> MSTLIPPPSKKQKKEAQLPREVAIIPKDLPNVSIKFQALDTGDNVGGALRVPGAISEKQLEELLNQLNGTSDDPVPYTFSCTIQGKKASDPVKTIDITDNLYSSLIKPGYNSTEDQITLLYTPRAVFKVKPVTRSSSAIAGHGSTILCSAFAPHTSSRMVTGAGDNTARIWDCDTQTPMHTLKGHYNWVLCVSWSPDGEVIATGSMDNTIRLWDPKSGQCLGDALRGHSKWITSLSWEPIHLVKPGSKPRLASSSKDGTIKIWDTVSRVCQYTMSGHTNSVSCVKWGGQGLLYSGSHDRTVRVWDINSQGRCINILKSHAHWVNHLSLSTDYALRIGAFDHTGKKPSTPEE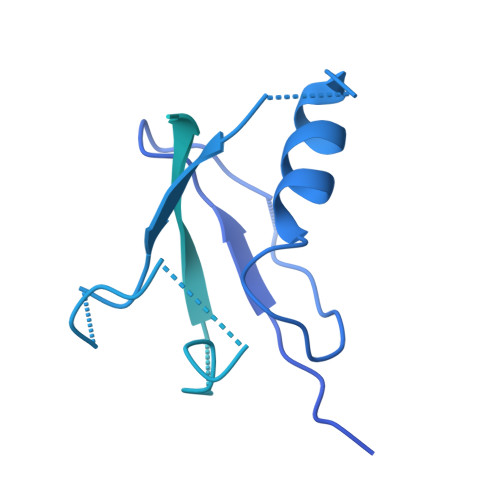AQKKALENYEKICKKNGNSEEMMVTASDDYTMFLWNPLKSTKPIARMTGHQKLVNHVAFSPDGRYIVSASFDNSIKLWDGRDGKFISTFRGHVASVYQVAWSSDCRLLVSCSKDTTLKVWDVRTRKLSVDLPGHKDEVYTVDWSVDGKRVCSGGKDKMVRLWTH>RRTYTLADYLKNTFRVKSYSLRWVSDSEYLYKQENNILLFNAEHGNSSIFLENSTFEIFGDSISDYSVSPDRLFVLLEYNYVKQWRHSYTASYSIYDLNKRQLITEEKIPNNTQWITWSQEGHKLAYVWKNDIYVKIEPHLPSHRITSTGKENVIFNGINDWVYEEEIFGAYSALWWSPNGTFLAYAQFNDTGVPLIEYSFYSDESLQYPKTVWIPYPKAGAVNPTVKFFIVNTDSLSSTTTTIPMQITAPASVTTGDHYLCDVAWVSEDRISLQWLRRIQNYSVMAICDYDKTTLVWNCPTTQEHIETSATGWCGRFRPAEPHFTSDGSSFYK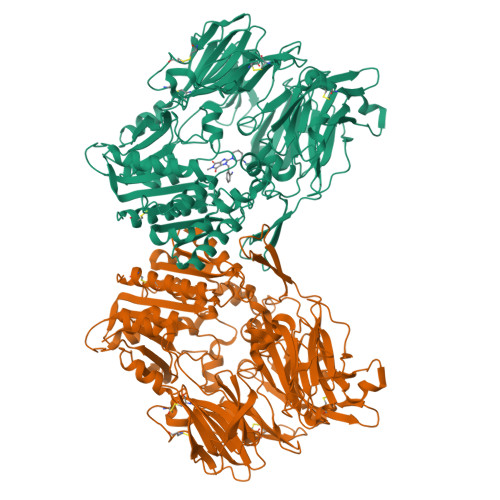IVSDKDGYKHICQFQKDRKPEQVCTFITKGAWEVISIEALTSDYLYYISNEYKEMPGGRNLYKIQLTDHTNKKCLSCDLNPERCQYYSVSLSKEAKYYQLGCRGPGLPLYTLHRSTDQKELRVLEDNSALDKMLQDVQMPSKKLDFIVLNETRFWYQMILPPHFDKSKKYPLLIDVYAGPCSQKADAAFRLNWATYLASTENIIVASFDGRGSGYQGDKIMHAINKRLGTLEVEDQIEAARQFLKMGFVDSKRVAIWGWSYGGYVTSMVLGSGSGVFKCGIAVAPVSRWEYYDSVYTERYMGLPTPEDNLDHYRNSTVMSRAENFKQVEYLLIHGTADDNVHFQQSAQISKALVDAGVDFQAMWYTDEDHGIASSTAHQHIYSHMSHFLQQCFSLR[2x]>[4x]TYCVGIRLDEGLVFASDSRTNAGVDNISTFRKMHVFEVPGERVIVLLTAGNLATTQAVISLLEERLKDPEERL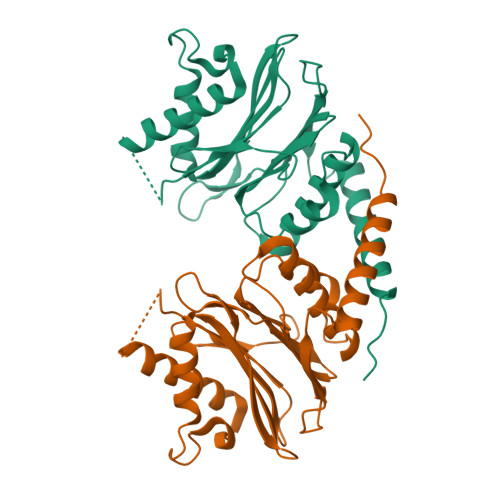LTAPSMFEAARLVGEALREVQARDAPALEADGVDFNASFILGGQIAGEPPRLFLIYPAGNFIEATPDTPFFQIGETKYGKPILDRVITPDTSLEDAAKCALVSFDSTMRSNLSVGLPLDLLVYERDSLRVGHRRRIDEDDPYFRMLRKQWSEGLRQAFDSLPDPPWE> GSHMDKIKLLKAAFLQYCRKDLGHAQMVVDELFSSHSDLDSDSELDRAVTQISVDLMDDYPASDPRWAESVPEEAPGFSNTSLIILHQLEDKMKAHSFLMDFIHQVGLFGRLGSFPVRGTPMATRLLLCEHAEKLSAAIVLKNHHSRLSDLVNTAILIALNKREYEIPSNLTPADVFFREVSQVDTICECLLEHEEQVLRDAPMDSIEWAEVVINVNNILKDMLQAASHYRQNRNSLYRREESLEKEPEYVPWTATSGPGGIRTVIIRQHEIVLKVAYPQADSNLRNIVTEQLVALIDCFLDGYVSQLKSVDKSSNRERYDNLEMEYLQKRSDLL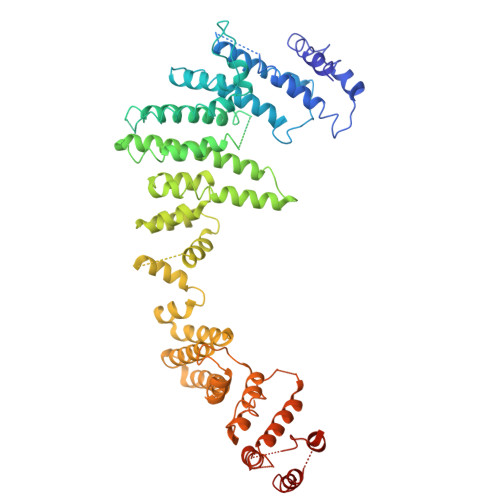SPLLSLGQYLWAASLAEKYCDFDILVQMCEQTDNQSRLQRYMTQFADQNFSDFLFRWYLEKGKRGKLLSQPISQHGQLANFLQAHEHLSWLHEINSQELEKAHATLLGLANMETRYFAKKKTLLGLSKLAALASDFSEDMLQEKIEEMAEQERFLLHQETLPEQLLAEKQLNLSAMPVLTAPQLIGLYICEENRRANEYDFKKALDLLEYIDEEEDININDLKLEILCKALQRDNWSSSDGKDDPIEVSKDSIFVKILQKLLKDGIQLSEYLPEVKDLLQADQLGSLKSNPYFEFVLKANYEYYVQGQI>[4x]SNAMNVNQIVRIIPTLKANNRKL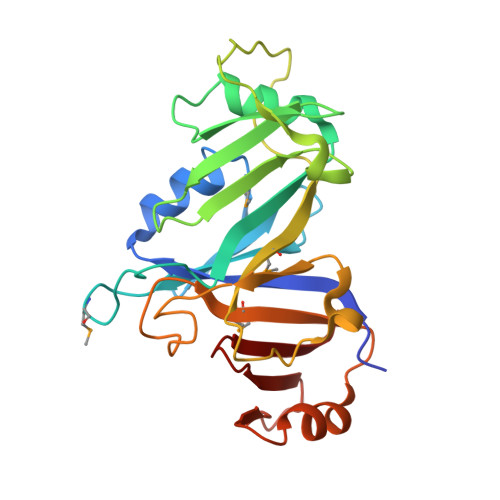NETFYIETLGMKALLEESAFLSLGDQTGLEKLVLEEAPSMRTRKVEGRKKLARLIVKVENPLEIEGILSKTDSIHRLYKGQNGYAFEIFSPEDDLILIHAEDDIASLVEVGEKPEFQTDLASISLSKFEISMELHLPTDIESFLESSEIGASLDFIPAQGQDLTVDNTVTWDLSMLKFLVNELDIASLRQKFESTEYFIPKSEKFFLGKDRNNVELWFEEV> MLGFNQDEYLTSAREIIAARQKAEQVADEIYQAGFSSLFFASVGGSLAPMMAINEFAKELTTLPVYVEQAAELIHKGNKRLNKDSVVITLSKSGDTKESVAIAEWCKAQGIRVVAITKNADSPLAQAATWHIPMRHKNGVEYEYMLLYWLFFRVLSRNNEFTSYDRFASQLEILTANLLKAKQKFDPQADAIASRYHNSDYMMWVGGAEMWGEVYLFSMCILEEMQWKRTRPVSSAEFFHGALELLEKDVPLILVKGEGKCRALDERVERFASKI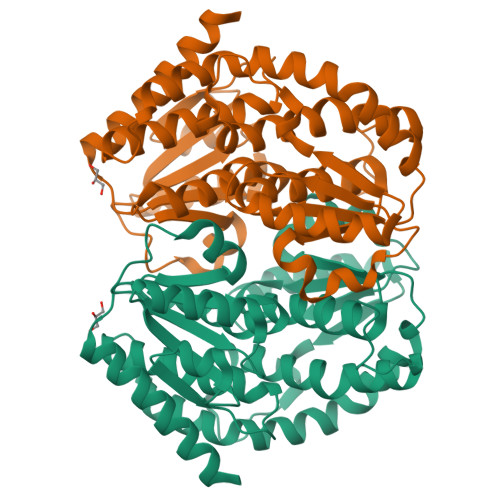TDNLVVIDPKAYALDGIDDEFRWIMAPCVVSTLLVDRLAAHFEKYTGHSLDIRRYYRQFDY> MTVTRRHFLKLSAGAAVAGAFTGLGLSLAPTVARAELQKLQWAKQTTSICCYCAVGCGLIVHTAKDGQGRAVNVEGDPDHPINEGSLCPKGASIFQLGENDQRGTQPLYRAPFSDTWKPVTWDFALTEIAKRIKKTRDASFTEKNAAGDLVNRTEAIASFGSAAMDN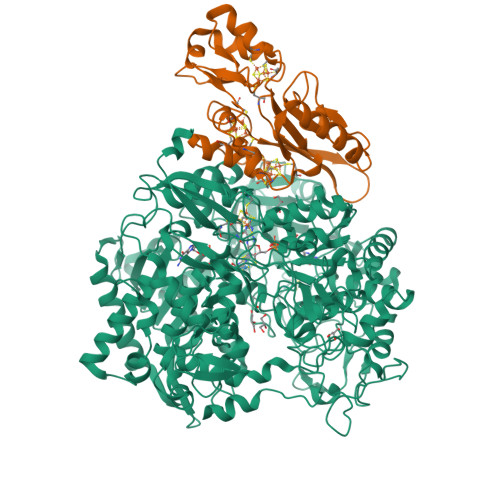EECWAYGNILRSLGLVYIEHQARIUHSPTVPALAESFGRGAMTNHWNDLANSDCILIMGSNAAENHPIAFKWVLRAKDKGATLIHVDPRFTRTSARCDVYAPIRSGADIPFLGGLIKYILDNKLYFTDYVREYTNASLIVGEKFSFKDGLFSGYDAANKKYDKSMWAFELDANGVPKRDPALKHPRCVINLLKKHYERYNLDKVAAITGTSKEQLQQVYKAYAATGKPDKAGTIMYAMGWTQHSVGVQNIRAMAMIQLLLGNIGVAGGGVNALRGESNVQGSTDQGLLAHIWPGYNPVPNSKAATLELYNAATPQSKDPMSVNWWQNRPKYVASYLKALYPDEEPAAAYDYLPRIDAGRKLTDYFWLNIFEKMDKGEFKGLFAWGMNPACGGANANKNRKAMGKLEWLVNVNLFENETSSFWKGPGMNPAEIGTEVFFLPCCVSIEKEGSVANSGRWMQWRYRGPKPYAETKPDGDIMLDMFKKVRELYAKEGGAYPAPIAKLNIADWEEHNEFSPTKVAKLMNGYFLKDTEVGGKQFKKGQQVPSFAFLTADGSTCSGNWLHAGSFTDAGNLMARRDKTQTPEQARIGLFPNWSFCWPVNRRILYNRASVDKTGKPWNPAKAVIEWKDGKWVGDVVDGGGDPGTKHPFIMQTHGFGALYGPGREEGPFPEHYEPLECPVSKNPFSKQLHNPVAFQIEGEKKAVCDPRYPFIGTTYRVTEHWQTGLMTRRCAWLVEAEPQIFCEISKELAKLRGIGNGDTVKVSSLRGALEAVAIVTERIRPFKIEGVDVHMVGLPWHYGWMVPKNGGDTANLLTPSAGDPNTGIPETKAFMVDVRKV;> MGKMFFVDLSRCTACRGCQIACKQWKNLPAEETRNTGSHQNPPDLSYVTLKTVRFTEKSRKGPGIDWLFFPEQCRHCVEPPCKGQADVDLEGAVVKDETTGAVLFTELTAKVDGESVRSACPYDIPRIDPVTKRLSKCDMCNDRVQNGLLPACVKTCPTGTMNFGDEQEMLALAEKRLAEVKKTYPGAVLGDPNDVRVVYLFTRDPKDFYEHAVADLAPSMMTRQQLFARLFRPRA>GPELVMRRGEIWQVDLDPARGSEANNQRPAVVVSNDRANATATRLGRGVITVVPVTSNIAKVYPFQVLLSATTTGLQVDCKAQAEQIRSIATERLLRPIGRVSAAELAQLDEALKLHLDLWS[2x];> TLED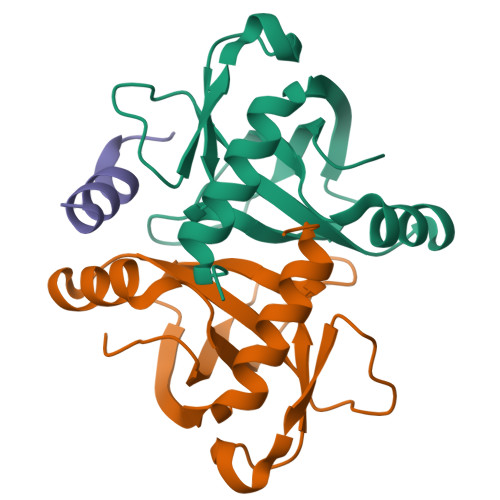DYANAWQEWSAAG>SNAASEKQQLSIEAARLYYQSDYSQQQIAEQLNISRPTVSRLLQYAKEKGYVQIRVM[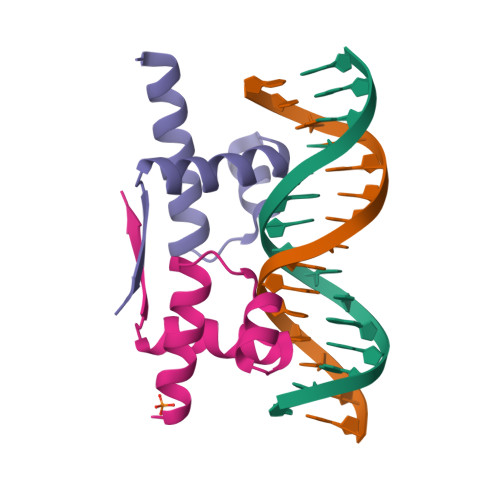3x]> SSQIRQNYSTEVEAAVNRLVNLYLRASYTYLSLGFYFDRDDVALEGVCHFFRELAEEKREGAERLLKMQNQRGGRALFQDLQKPSQDEWGTTLDAMKAAIVLEKSLNQALLDLHVLGSAQADPHLCDFLESHFLDEEVKLIKKMGDHLTNIQRLVG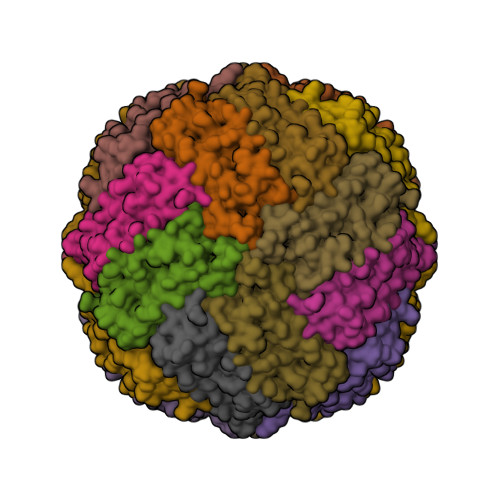SQAGLGEYLFERLTLKHD> GSHMTWLSDFPQAWAETGGMGLAVRQAPLIIPLKATSTPVSIKQYPMSQEARLGIKPHIQRLLDQGILVPCQSPWNTPLLPVKKPGTNDYRPVQDLREVNKRVEDIHPTVPNPYNLLSGLPPSHQWYTVLDLKDAFFCLRLHPTSQPLFAFEWRDPEMGISGQLTWTRLPQGFKNSPTLFDEALHRDLADFRIQHPDLILLQYVDDLLLAATSELDCQQGTRALLQTLGNLGYRASAKKAQICQKQVKYLGYLLKEGQRWLTEARKETVMGQPTPKTPRQLREFLGTAGFCRLWIPGFAEMAAPLYPLTKTGTLFNWGPDQQKAYQEIKQALLTAPALGLPDLTKPFELFVDEKQGYAKGVLTQKLGPWRRPVAYLSKKLDPVAAGWPPCLRMVAAIAVLTKDAGKLTM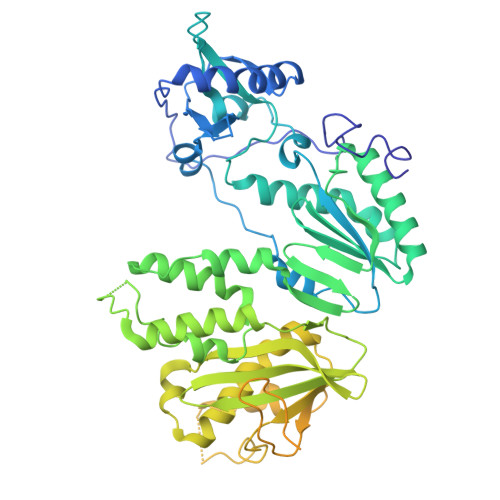GQPLVIKAPHAVEALVKQPPDRWLSNARMTHYQALLLDTDRVQFGPVVALNPATLLPLPEEGLQHNCLDILAEAHGTRPDLTDQPLPDADHTWYTDGSSLLQEGQRKAGAAVTTETEVIWAKALPAGTSAQRAELIALTQALKMAEGKKLNVYTDSRYAFATAHIHGEIYRRRGLLTSEGKEIKNKDEILALLKALFLPKRLSIIHCPGHQKGHSAEARGNRMADQAARKAAITETPDTSTLL4-iodanyl-3~{H}-pyridin-2-one | C5 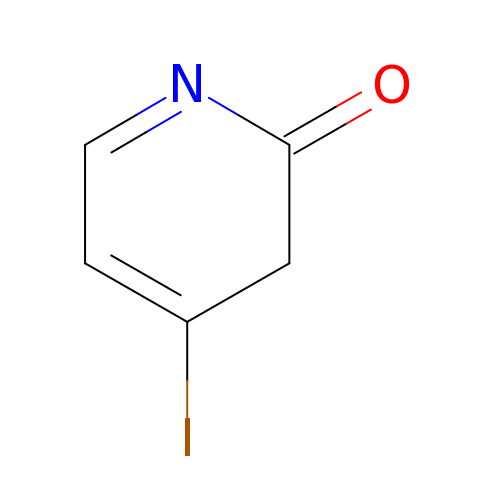H4 I N O | GRVSGGNZRNHMQI-UHFFFAOYSA-N(1S,4R,7AR)-4-BUTOXY-1-[(1R)-1-FORMYLPROPYL]-2,4,5,6,7,7A-HEXAHYDRO-1H-ISOINDOLE-3-CARBOXYLIC ACID | C17 H27 N O4 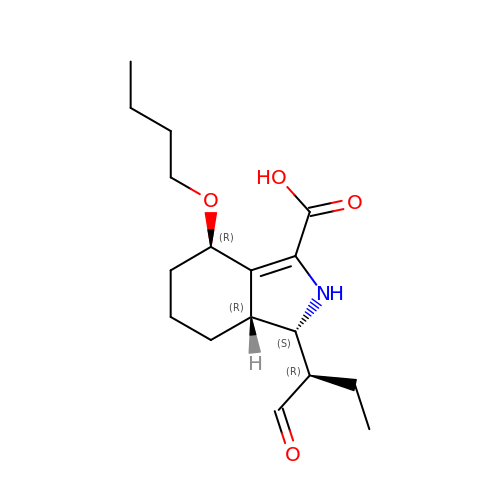| WRBRCIHZCYLBFW-KYEXWDHISA-N>[3x]VINLDMIKASYITMGYDKNAAEVGEIIKATVKINKITNFSGYQVNIKYDPTVLQAVNPKT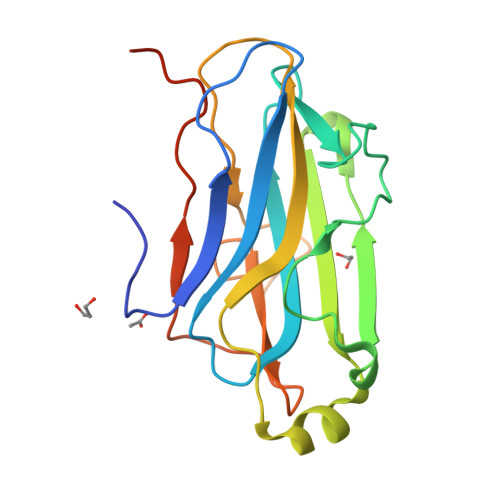GVAYTNSSLPTSGELLVSEDYGPIVQGVHKISEGILNLSRSYTALEVYRASESPEETGTLAVVGFKVLQKKATTVVFEDSETMPNGITGTTLFNWYGNRIQSGYFVIQPGEINSAPIATLEHHHHHH>[2x]MTQPLVGKQILIVEDEQVFRSLLDSWFSSLGATTVLAADGVDALELLGGFTPDLMICDIAMPRMNGLKLLEHIRNRGDQTPVLVISATENMADIAKALRLGVEDVLLKPVKDLNRLREMVFACLYPSMFNSRVEEEERLFRDWDAMVDNPAAAAKLLQELQPPVQQVISHCRVNYRQLVAADKPGLVLDIAALSENDLAFYCLDVTRAGHNGVLAALLLRALFNGLLQEQLAHQNQRLPELGALLKQVNHLLRQANLPGQFPLLVGYYHRELKNLILVSAGLNATLNTGEHQVQISNGVPLGTLGNAYLNQLSQRCDAWQCQIWGTGGRLRLMLSAE

In the case of σs, a specialized adaptor protein RssB, also referred to as SprE, is not only required for direct recognition of the substrate but also required for its preparation and delivery to the AAA+ protease, ClpXP. RssB is a response regulator (RR), and as such is composed of an N-terminal receiver (REC) domain and a C-terminal output domain (also known as an effector domain). In contrast to most RRs (which contain a DNA binding domain) RssB is linked to a protein binding domain, and as such represents one of the small groups of RRs (~1% of all RRs). Nevertheless, like most RRs, RssB is phosphorylated on a conserved Asp residue (Asp58) within the N-terminal REC domain.

Overall, the structure consists of five repetitive (αβ)-elements which form a parallel β-sheet (β2–β1–β3–β4–β5–) sandwiched by two helices (α1 and α5) on one side and three helices (α2–α4) on the opposite side. Similar to several REC domains, our structure of RssBN formed a dimer in the asymmetric unit. However, in contrast to many RRs the RssBN dimer showed an anti-parallel orientation, which is mainly stabilized by β-strand augmentation via the terminal β2-strands. This orientation is different to the biologically active dimer of several RRs including PhoP from E. coli. Superposition of RssBN onto the RssB/IraD structure revealed an r.m.s.d. of 1.4 Å. While the core structure of this domain is well preserved (with the exception of small deviations around Asp58), there were clear changes in the conformation of the α5 helix across the structures. From analysis of the B-factors of RssBN (which resemble molecular flexibility) it became obvious that the last helix (α5), in particular, shows higher mobility. This is supported by the observation of limited hydrophobic contacts between this helix and the core domain structure. Significantly, Arg117 is located on the mobile α5 helix of RssBN, which is directly linked to the C-terminal domain that makes direct contact to σs. Based on our mutational analysis of conserved residues located within the N-domain, we propose that phosphorylation of RssB (at Asp58) is sensed by the conserved residue (Lys108) located within the 4-5-5 interface.>[2x]MSALFEPYTLKDVTLRNRIAIPPMCQYMAEDGLINDWHQVHYASMARGGAGLLVVEATAVAPEGRITPGCAGIWSDAHAQAFVPVVQAIKAAGSVPGIQIAHAGRKASANRPWEGDDHIGADDARGWETIAPSAIAFGAHLPNVPRAMTLDDIARVKQDFVDAARRARDAGFEWIELHFAHGYLGQ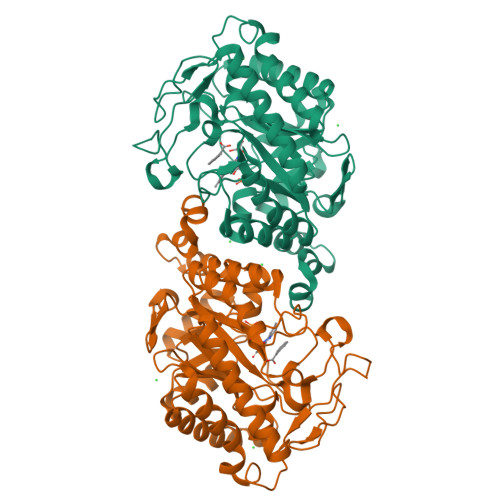SFFSEHSNKRTDAYGGSFDNRSRFLLETLAAVREVWPENLPLTARFGVLEYDGRDEQTLEESIELARRFKAGGLDLLSVSVGFTIPETNIPWGPAFMGPIAERVRREAKLPVTSAWGFGTPQLAEAALQANQLDLVSVGRAHLADPHWAYFAAKELGVEKASWTLPAPYAHWLERYRLEHHHHHH> SPSVEACGYSDRLKQITIGNSTITTQDSLHTVLAYGEWPTYLSDIDATSVDKPTHPE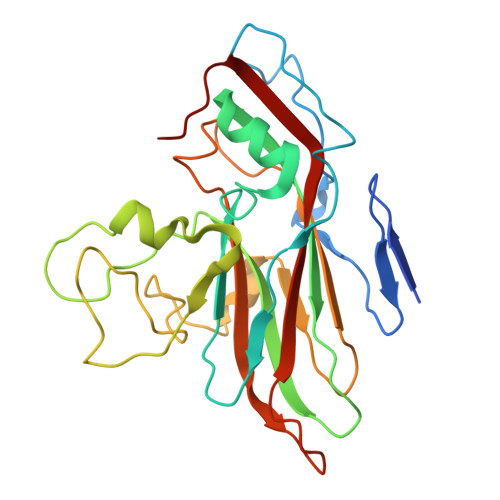TSADRFYTLDSVEWQVGSHGWWWKLPDALKDMGVFGQNMYYHSMGRSGFIIHTQCNATKFHSGALIVAVIPEHQLAYVGGVKVNVGYDHTHPGQSGHQIRGPSQSNDRSGGKPDEDPLFNCNGTLLGNITIFPHQIINLRTNNSSTIVVPYINCVPMDNMLKHNNLSLVIIPLVPLRPGSSGINSVPITVTIAPYKSEFSGAMEAQRQ>IQIREYKRCGQDEERVRRECKERGERQNCHYV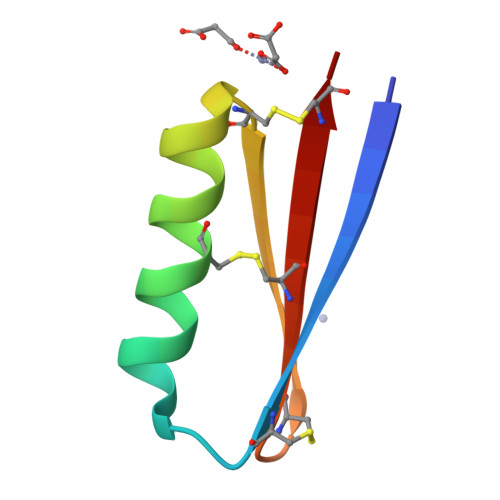IHKEGNCYVCGIICW[2x]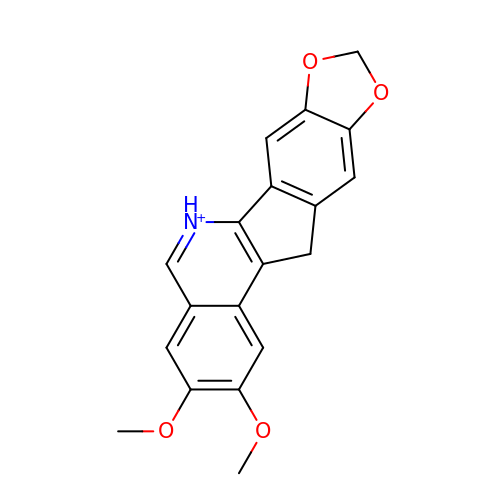2,3-DIMETHOXY-12H-[1,3]DIOXOLO[5,6]INDENO[1,2-C]ISOQUINOLIN-6-IUM | C19 H16 N O4 | LXDREMZQGAILJU-UHFFFAOYSA-O(2S,3S)-2-(3,4-DIHYDROXYPHENYL)-3,5,7-TRIHYDROXY-2,3-DIHYDRO-4H-CHROMEN-4-ONE | C15 H12 O7 | 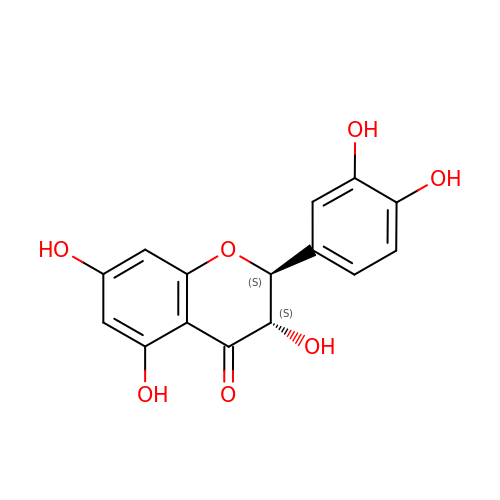CXQWRCVTCMQVQX-CABCVRRESA-N>AGAGAGATGGGTGCGTT[2x]

Herein we further expand the structure and sequence complexity of DNA four-stranded architecture by presenting a high-resolution crystal structure of DNA1 (5′- AGAGAGATGGGTGCGTT-3′). This is the first DNA structure that contains all the internal A-, G-, C-, T-tetrads, A:T:A:T tetrads, bulged nucleotides and multiple metal ions including Li+, NH4+, Na+ and Pb2+ in one single structure. Though it contains only one GGG motif, DNA1 can form parallel quadruplex. Our site-specific mutagenesis and biophysical studies showed that the central ATGGG motif of DNA1 plays important role in the quadruplex formation.

Though 8–17 DNAzyme was present in the crystallization sample, only DNA1 sequence crystallized out under the conditions composed of 100 mM CAPS-NaOH pH 10.5, 200 mM Li2SO4 and 2.0 M (NH4)2SO4; the crystal diffracts to 1.45 Å resolution. The crystal belongs to P21212 space group, it contains two DNA1 molecules per asymmetric unit. Via the 2-fold symmetry along the long axis, DNA1 can assemble into quadruplex with four DNA strands parallelly orientated. The central region (G2–G15) of DNA1 forms 13 homogenetic tetrads stacking on each other, which are the longest continuous tetrads observed within single quadruplex structure. However, even though all the thymine and cytosine residues in DNA1 form tetrads, the middle A7 residues form a kink in our structure. As one of the most common cofactors of G4, Na+ ion accounts for the majority cations bound in the DNA1 structure. One well-defined Pb2+ ion is captured in our DNA1 structure, representing the first quadruplex–Pb2+ complex structure. The Pb2+ is bound in-between the G13-tetrad and the C14-tetrad with eight coordination form. The very weak electron density suggests that it is one Li+ ion bound in-between the G15 and A1*:T16:A1*:T16 tetrads. As a result, multiple DNA1 quadruplexes assemble into an infinite nanowire-like structure, which captures one cation in-between each tetrad layer.> SFSQAVSGLNAAATNLDVIGNNIANSATYGFKSGTASFADMFAGSKVGLGVKVAGITQDFTDGTTTNTGRGLDVAISQNGFF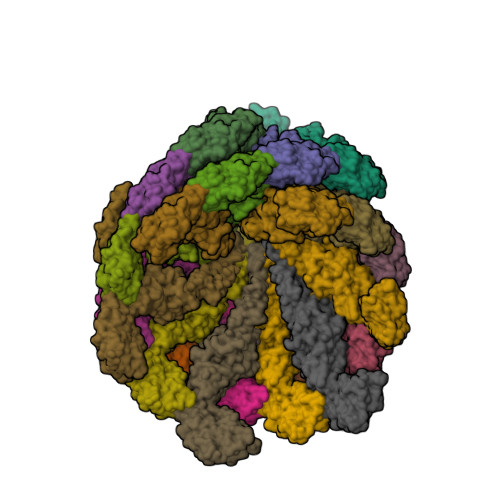RLVDSNGSVFYSRNGQFKLDENRNLVNMQGMQLTGYPATGTPPTIQQGANPAPITIPNTLMAAKSTTTASMQINLNSTDPVPSKTPFSVSDADSYNKKGTVTVYDSQGNAHDMNVYFVKTKDNEWAVYTHDSSDPAATAPTTASTTLKFNENGILESGGTVNITTGTINGATAATFSLSFLNSMQQNTGANNIVATNQNGYKPGDLVSYQINNDGTVVGNYSNEQEQVLGQIVLANFANNEGLASQGDNVWAATQASGVALLGTAGSGNFGKLTNGALEASNVDLSKELVNMIVAQRNYQSNAQTIKTQDQILNTLVNLR> MKDTIALVVSTLNNPFFVSLKDGAQKEADKLGYNLVVLDSQNNPAKELANVQDLTVRGVKILLINPVDSDAVGNAVKMANQANIPVITLDRQATKGEVVSHIASDNVLGGKIAGDYIAKKAGEGAKVIELQGIAGTSAARERGEGFQQAVAAHKFNVLASQPADFDRIKGLNVMQNLLTAHPDVQAVFAQNDEMALGALRALQTAGKSDVMVVGFDGTPDGEKAVNDGKLAATIAQLP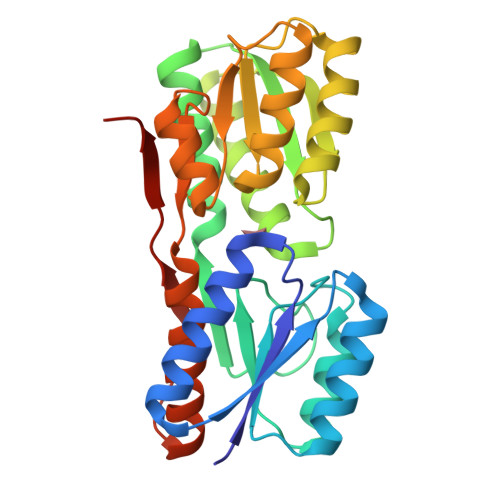DQIGAKGVEVADKVLKGEKVQAKYPVDLKLVVKQHHHHHH> GIDPFTKMTRPSSDLTAFREHFAKAKHIAIITGAGVSAESGVPTFRGPGGFWRKWQAQDLATPEAFSRDPSLVWEFYHYRREVMRSKMPNPAHLAIAECEARLGQQGRSVVIITQNIDELHHRAGSKHVYEIHGSLFKTRCMSCGEVKANHKSPICPALDGKGAPDPNTKEARIPVELLPRCERKSCNGLLRPHVVWFGETLDSDILTAVERELEKCDLCLVVGTSSIVYPAAMFAPQVASRGVPVAEFNMECTPATQRF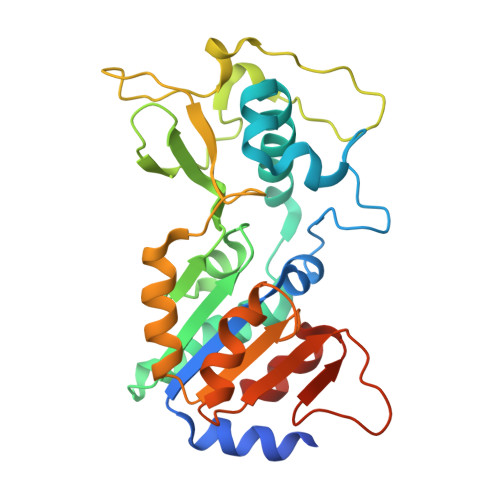KYHFEGPCGSTLPPALERHESEAV We describe here the use of an artificial cofactor employing the well‐known biotin‐streptavidin system to catalyze a Baylis‐Hillman reaction. As protein host, we chose streptavidin, as it can be easily crystallized and thereby supports the design process. There are several examples using streptavidin as the host for these cofactors, since its natural ligand biotin binds strongly (K d∼10−15 M) and is easy to modify with catalysts at the carboxylic acid group. No enzyme is known to naturally catalyze the Baylis‐Hillman reaction, a very versatile and atom‐economic C−C bond forming reaction for the production of various functionalized compounds and intermediates of active pharmaceutical ingredients (APIs).

We chose a derivative of DMAP as the artificial cofactor due to its low steric demand, which will facilitate its inclusion into the protein scaffold. The protein host around the cofactor was rationally designed on the basis of high‐resolution crystal structures obtained after each variation of the amino acid sequence. The location of the catalyst is in a shallow cavity at the surface of the protein. The system was evolved through repeated cycles of mutagenesis, activity tests, and structure determination. According to the presented structures and calculations the catalytically active site is too shallow to undergo interactions with 1.

> MASMTGGQQMGRDEAGITGTWYNQLGSTFIVTAGADGALTGTYESAAGKAESRYVLTGRYDSAPATDGSGTALGWTVAWKNNYRNAHSATTWSGQYVGGAEARINTQWLLTAGQTEANGWASTLVGHDTFTKVKPSAASIDAAKKAGVNNGNPLDAVQQ Prochlorococcus marinus MIT 9313, a typical Cyanobacteria, contains an ABC-type transporter, UrtABCDE, which may account for the transport of urea. UrtABCDE consists of three parts: a substrate-binding protein (UrtA) located in the periplasm, two hydrophobic transmembrane domains (UrtB and UrtC), and two hydrophilic nucleotide-binding domains (UrtD and UrtE). UrtA possesses the typical structural characteristics of cluster B-Ⅱ extracellular substrate-binding proteins. It consists of two domains, an N-terminal domain (NTD) and a C-terminal domain (CTD), linked by a hinge region.

The crystal of UrtA/urea complex belongs to the P21 space group and was solved to 1.60 Å. The structure of UrtA/urea complex shows that each asymmetric unit contains one UrtA molecule. The electron density map of the UrtA/urea complex structure shows that a single urea molecule is tightly bound to the hinge region between the two domains, interacting mainly with the residues in the hinge. Compared to the other three types of UTs, UrtA exhibits a strong urea binding affinity, with a Kd of 141.3 ± 11.2 nM. The six hydrogen bonds formed between urea and Ser122, Gln144, Tyr190, and Asn246 constituted a stable binding plane. Mutation on any of these four amino acid residues resulted in a significant decrease or complete loss of the urea binding affinity. The effect of Trp120 on urea binding may be attributed to the formation of hydrogen bond between the side chain of Trp120 and Asn246, which stabilizes the position of Asn246, a key residue involved in urea binding. In the UrtA/urea structure, the binding pocket was present in a closed state, and no entrance was found. Thus, we proposed that apo UrtA without binding urea contains a urea entrance and will undergo a similar closing process as other cluster B-Ⅱ proteins. Consistent with other cluster B-Ⅱ proteins, the conformational change of UrtA without urea is like a “Venus Flytrap”. These results suggested that UrtA undergoes a similar process to the typical cluster B-Ⅱ proteins, in which a urea molecule enters the binding site through the entrance aside the hinge region and causes apo UrtA to close around the urea molecule.

> MCGGGSDKTANTDFDDTVTVGILHSLSGTMAISESTLVDTEKMAIEEINAAGGVEVDGKKYKIDYIVEDGASDWPTFAEKSKKLIDQDSVPVVFGGWTSASRKAMLPVYESKNAFLYYPIQYEGQECSNNIFYTGATPNQQSEPATKFMFEKSPAAGKPFFLVGSDYVFPRTSNTITKEQVKALGGKVVGEDYLPLGNTEVAPIIAKIKKALPDGGVIINTLNGDQNVAFFKQIQDAGLTPENGYYVMSYSIAEEEISTIGPEFLEGHYGAWNYMMSIDTPASKKFASDFKAKYGNDRQVADPQESAYNMVYLWKAAVEKANSFDDDKVREALIGIEFDAPQGPVKVMPNHHLSQTVRIGKITKDGQFEILEETDGPVAPQAWNQFEPSSKGYACDWTDANKGEKYKLHHHHHH>EELQKSIGHKPEPTDEEWELIKTVTEAHVATNAQGSHWKQKRKFLPEDIGQAPIVNAPEGGKVDLEAFSHFTKIITPAITRVVDFAKKLPMFCELPCEDQIILLKGCCMEIMSLRAAVRYDPESETLTLNGEMAVTRGQLKNGGLGVVSDAIFDLGMSLSSFNLDDTEVALLQAVLLMSSDRPGLACVERIEKYQDSFLLAFEHYINYRKHHVTHFWPKLLMKVTDLRMIGACHA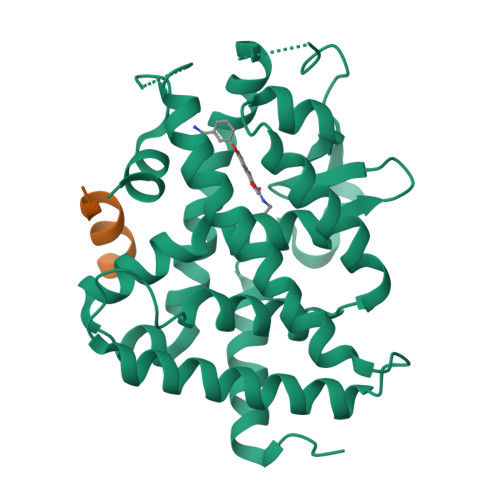SRFLHMKVECPTELFPPLFLEVFED[2x];>ENALLRYLLDKD[2x]> MAVPDQKSPNVLLQNLCCRILGKGEADVAQQFQYAVRVIGSNFAPTVERDEFLVTEKIKKEFVRQRREADGALFSELHRKLQSQGVLKNRWSILYLLLSLSEDPRKQPNKTSSFAALFAQALPRDAHSTPYYYARPQSLPLSYQDRNVQCAQNAASIGSSGISSIGMYALNGPTPQSIIQGQSNQTPNMGDALRQQLGSRLAWTLAAGQQPSQQSTTTKGLPNTVSRNVPRTRREGDSSGSVEITETSLVRDLLYVFQGIDGKFVKMCNSENCYKVDGKVAVSKSLKDITSKLSELGWLHNKIKKYTDQRSLDRAFGLVGQSFCAALHQELKEYYRLLSVLHSQLQVEDDQGVNLGVESSLTLRRLLVWTFDPKIRLKTLAALVDHCQGRKGGELASAVHAYTKTGDPYMRSLVQHILGLVAYPILNFLYRWIYDGELEDTYHEFFVASDPVVKTDRLWHDKYSLRKSMIPSFMTMDQSRKVLLIGKSINFLHQVCHDQTPASKAMAVGKSAESPKDAAELFTDLENAFQTKIDAAYFDTSKYLLDVLNKNYNLLEHMQAMRRYLLLGQGDFIRHLMDLLKPELVRPATTLYQHNLTGILETAVRATNAQFDNPEILKRLDVRLLEVSPGDTGWDVFSLDYHVDGPIATVFTRECMSHYLRVFNFLWRAKRMEYILTDIWKGHMCNAKLLKGMPELSGVLHQCHILASEMVHFIHQMQYYITFEVLECSWDELWNKVLKAQDLDHIIAAHDVFLDTIISRCLLDSESRALLNQLRAVFDQIIEFQNAQDALYRAALEELQQRLQFEERKKERESEGEWGVTAAEEDVENKRIQEFQESIPKMRSQLRILTHFYQGIVQQFLVLLTTSTDESL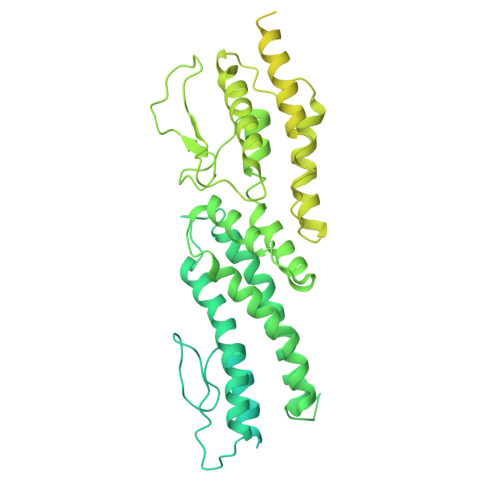RFLSFRLDFNEHYKAREPRLRVSMGTRGRRSFHV> EMVDNLRGKSGQGYYVEMTVGSPPQTLNILVDTGSSNFAVGAAPHPFLHRYYQRQLSSTYRDLRKGVYVPYTQGKWEGELGTDLVSIPHGPQVTVRANIAAITESDKFFIQGSNWEGILGLAYAEIARPDDSLEPFFDSLVKQTHVPNLFSLQLCGAGFPLQQSEVLASVGGSMIIGGIDHSLYTGSLWYTPIRREWYYEVIIVRVEINGQDLKMDCKEYNYDKSIVDSGTTNLRLPKKVFEAAVKSIKAASSTEKFPDGFWLGEQLVCWQAGTTPWNIFPVISLYLMGEVTQQSF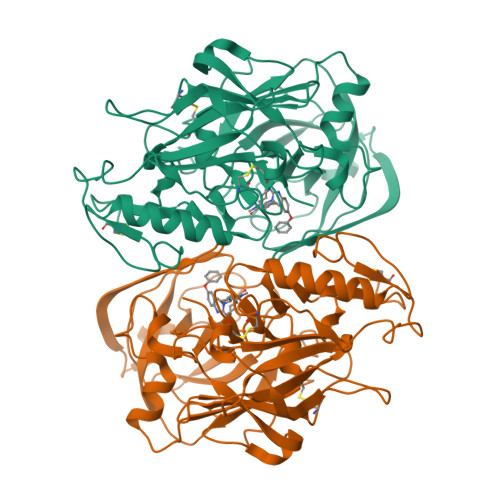RITILPQQYLRPVEDVATSQDDCYKFAISQSSTGTVMGAVIMEGFYVVFDRARKRIGFAVSACHVHDEFRTAAVEGPFVTLDMEDCGYN> PCVVGGQADTIYPAIANQMAHQMHEDAQTEASKRGLAKLRADAKQGIYKKNRKPQELSNICNITLQHSNDSRNGNNGGACTGKDGNNERFKIGTEWKIGEKVETTDTDAYIPPRR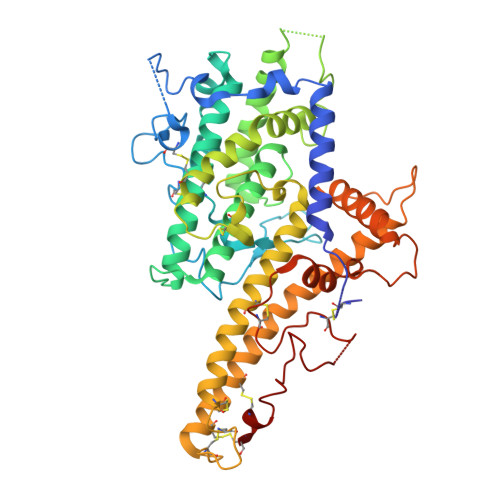QHMCTSNLENLNVSWVTEDGKAIHSLLGDVQLAAKMDADEIIKRYKKHNTLTDPIQQKDQESICRAVRYSFADLGDIIRGRDLWEHGDQTKLQGHLQIIFGKIKEEIKKKHPGINGNDKYKGDEKNNPPYKQLREDWWEANRHQVWRAMQCELKNLKKSNGDCHYNSRGTPLDDYIPQRLRWMVEWAEWFCKMQSQEYDKLMKQCSQCMSKGGDCRKGDVNCTSCEQACEEYKKKIKKWEKQWNKIKDKYEELYLQAKIAFAGTSFGGGDRDYQQMVHFFKELQKVTGDTTLGDTTSPYSTAAGYIHQEGHVDECTEQTQFCKNRNGNTASGKEDDNYTFKDPPPKYANACKCD> GSSMKASSGDQGSPPCFLRFPRPVRVVSGAEAELKCVVLGEPPPVVVWEKGGQQLAASERLSFPADGAEHGLLLTAALPTDAGVYVCRARNAAGEAYAAAAVTVLEPPA;> GSSRGIPPKIEALPSDISIDEGKVLTVACAFTGEPTPEVTWSCGGRKIHSQEQGRFHIENTDDLTTLIIMDVQKQDGGLYTL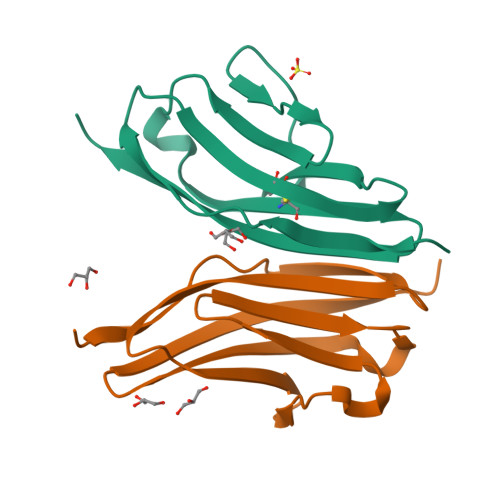SLGNEFGSDSATVNIHIRSI>MEICPAVKRDVDLFLTGTPDEYVEQVAQYKALPVVLENARILKNCVDAKMTEEDKENALSLLDKIYTSPLCVKMAETCPIFYDVFFAVANGNELLLDLSLTKVNATEPERTAMKKIQDCYVENGLISRVLDG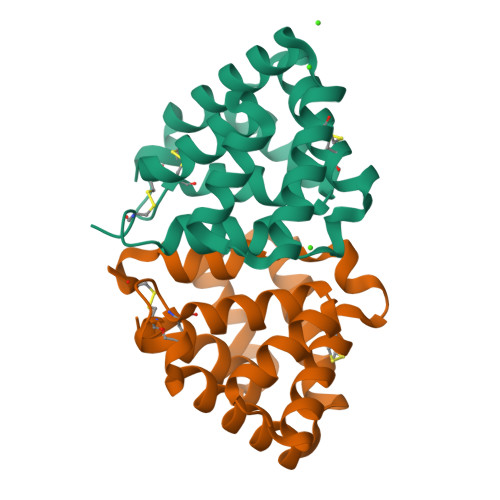LVMTTISSSKDCMGEHHHHHH[2x]> GYSA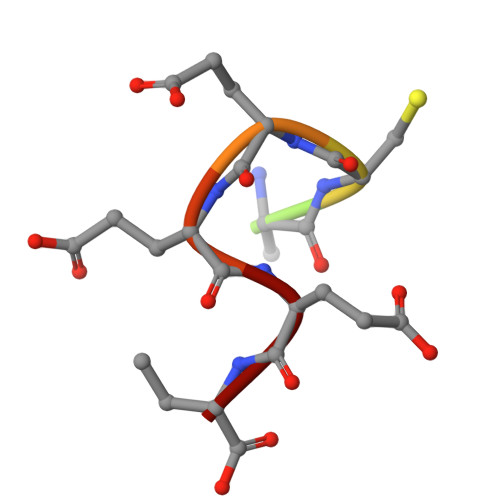CEEEN>GPHMGAYWMSPTADDIRAMNRMQRQRVVGFTVGRENVGSVQFKVPVDLSNINLDDLFGTIVILEPRSATVYPNAAKKPPMGKGLNVPALISLEHSWPRGGPTIKGRRLERHIERLKSIPDTTFESYDPETG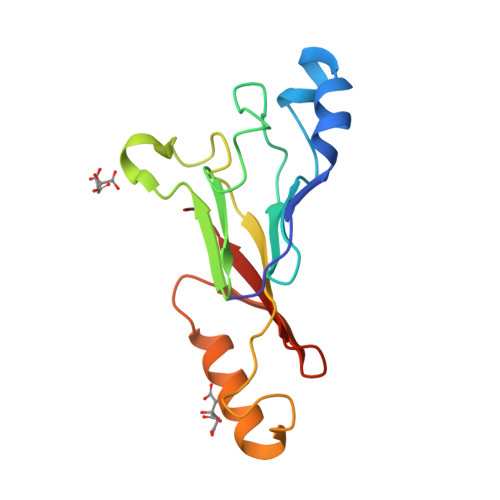VWAFSVEHF[2x]> SNARDPRPLRDKNFQSAIQEEIYDYLKKNKFDIETNHPISIKFLKQPTQKGFIIIFKWLYLRLDPGYGFTKSIENEIYQILKNLRYPFLESINKSQISAVGGSNWHKFLGMLHWMVRTNIKLDMCLNKVDRSLINQNTQEITILSQPL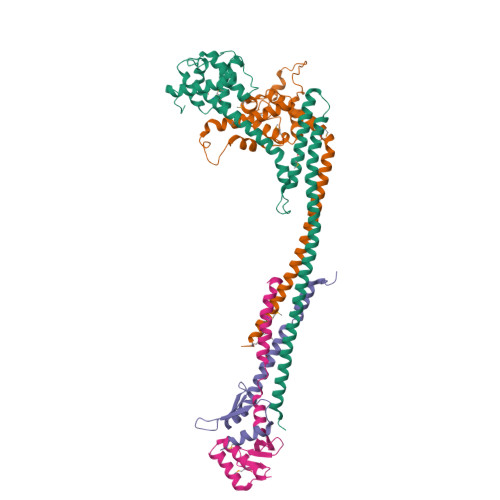KTLDEQDQRQERYELMVEKLLIDYFTESYKSFLKLEDNYEPSMQELKLGFEKFVHIINTDVTSTELKLEELKVDLNRKRYKLHQQVIHVIDITSKFKINIQSSLENSENELGNVIEELRNLEFETEHNV;> SNASIFKDLEALSFQSNASRNQDVFPILDLQELVICLQSCDFALATQENISRPTSDYMVTLYKQIIENFMGISVESLLNSSNQETGDGHLQEENENIYLDTLNVLVLNKICFKFFENIGVQDFNMTDLYKPEAQRTQRLLSAVVNYARFREERMFDCNSFILQMESLLGQINKLNDEIKQLQKDFEVEVKEIEIEYSLLSGHINKYMNEMLEYMQ;> MSQKDNLLDNPVEFLKEVRESFDIQQDVDAMKRIRHDLDVIKEESEARLKLYRSLGVILDLENDQVLINRKNDGNIDILPLDNNLSDFYKTKYIWERLGK;> MASIDAFSDLERRMDGFQKDVAQVLARQQNHVALYERLLQLRVLPGASDVHDVRFVFGDDSRCWIEVAMHGDHVIGNSHPALDPKSRATLEHVLTVQGDLAAFLVVARDMLLASL1,2-oxazole-5-carbothioamide | C4 H4 N2 O S | 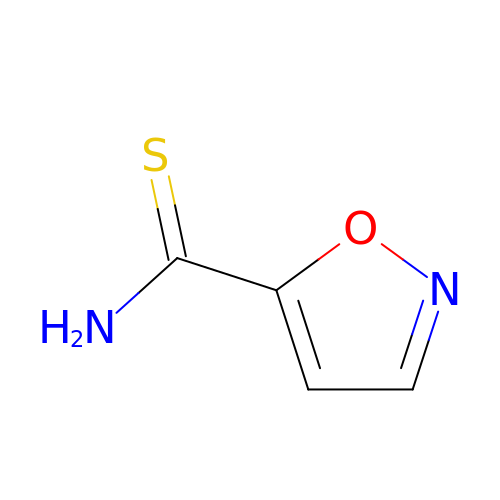CEDRGDFENMZKCQ-UHFFFAOYSA-N> MDKDEAWKQVEQLRREGATRIAYRSDDWRDLKEAWKKGADILIVDATDKDEAWKQVEQLRREGATEIAYRSDDWRDLKEAWKKGA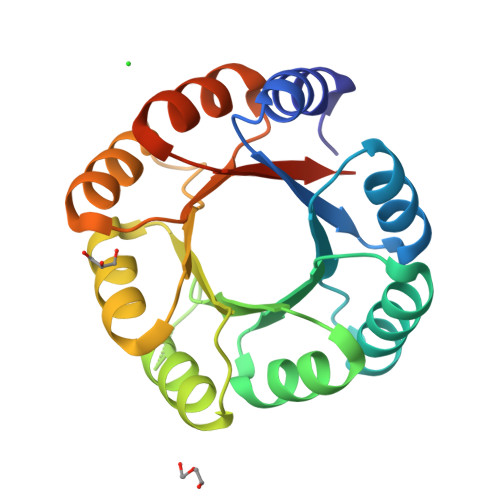DILIVDATDKDEAWKQVEQLRREGATRIAYRSDDWRDLKEAWKKGADILIVDATDKDEAWKQVEQLRREGATEIAYRSDDWRDLKEAWKKGADILIVDATGLEHHHHHH> GAGCCTGACTACA;> CGTGGACA;> TCTGTG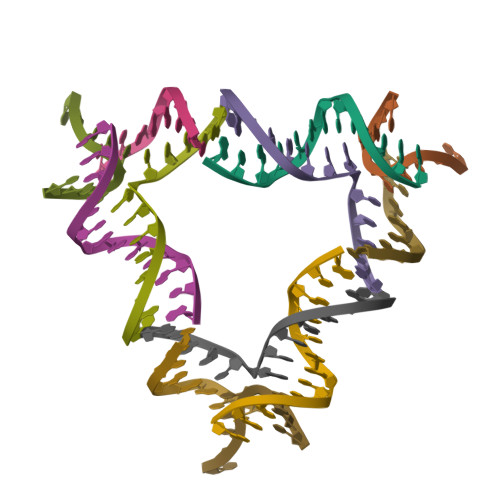GC;> TGTAGTCACCACG> GSMDLYRQSLEIISRYLREQATGAKDTKPMGRSGATSR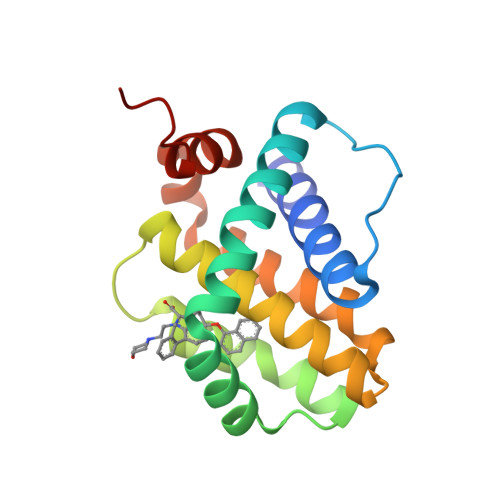KALETLRRVGDGVQRNHETAFQGMLRKLDIKNEDDVKSLSRVMIHVFSDGVTNWGRIVTLISFGAFVAKHLKTINQESCIEPLAESITDVLVRTKRDWLVKQRGWDGFVEFFHVEDLEG GerQ is a spore coat protein known for its importance in spore germination in B. subtilis and B. cereus. GerQ has been reported to function by recruiting CwlJ, a protein responsible for hydrolyzing the cortex peptidoglycan surrounding dormant spores and essential for Ca2+-DPA induced spore germination. The spores are enveloped by a proteinaceous, self-assembled, multilayered structure known as the spore coat. GerQ assembles into a structurally stable architecture consisting of rings containing nine subunits, which stacks to form filaments.

In this study, we re-process the previous cryo-EM data and successfully determine the structure of these 8 nm filaments at a resolution of 3.3 Å. The GerQ filament exhibits an overall structure characterized by stacked layers, with each layer composed of nine GerQ subunits that form a bowl-like shape. These layers are related to each other by helical symmetry with a rise of 34.2 Å and a twist of −18.4°. Within each layer, the nine GerQ subunits are related to each other with C9 point group symmetry. The filament core in a single GerQ subunit contains residues 91-169. It comprises two α-helixes, five β-strands, and connecting loops that link these secondary structures. The bowl-like structure formed by the nine subunits features a wide opening (∼39 Å) on one side and a narrow opening (~17 Å) on the other side. Each interface is formed by two adjacent GerQ subunits, where β-strands from both GerQ subunits create a continuous antiparallel β-sheet. The subunit-to-subunit interface is further stabilized by hydrophobic interactions and π-π stackings. In contrast to the tightly packed bowl-like structure, the interactions between two adjacent layers in the GerQ filament are relatively weak.

>MKPKKNQYQQMQGMGMGMDMQGFQPQLGPNPYPQPQGQGSQMMPMQQQMTMPMQQGQQGFGGGFPGQPQQQGGGSFQIPSGPSSSQNVPGMLPIEESYIENILRLNRGKTATIYMTFENSKEWNSKIFRGVIEAAGRDHIIISDPKTGTRYLLLTIYLDYITFDEEIAYTYPYSMSSYSPR[18x]>MRDLKGIFSALLVSFNEDGTINEKGLRQIIRHNIDKMKVDGLYVGGSTGENFMLSTEEKKEIFRIAKDEAKDQIALIAQVGSVNL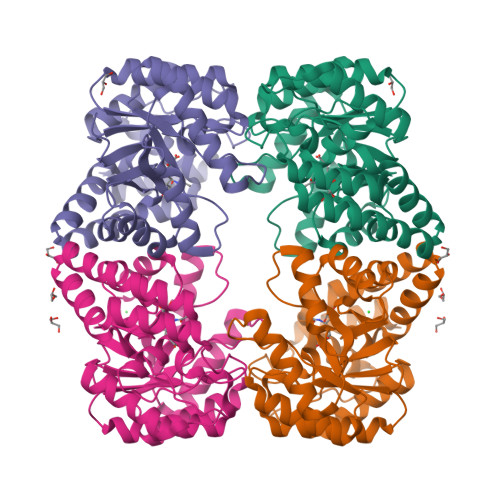KEAVELGKYATELGYDCLSAVTPFYYKFSFPEIKHYYDTIIAETGSNMIVYSIPFLTGVNMGIEQFGELYKNPKVLGVKFTAGDFYLLERLKKAYPNHLIWAGFDEMMLPAASLGVDGAIGSTFNVNGVRARQIFELTKAGKLKEALEIQHVTNDLIEGILANGLYLTIKELLKLEGVDAGYCREPMTSKATAEQVAKAKDLKAKFLS[2x]(1-{2-[bis(2-{4-[({(6R)-5-(acetylamino)-3,5-dideoxy-6-[(1R,2R)-1,2,3-trihydroxypropyl]-beta-L-threo-hex-2-ulopyranonosyl}oxy)methyl]-1H-1,2,3-triazol-1-yl}ethyl)amino]ethyl}-1H-1,2,3-triazol-4-yl)methyl 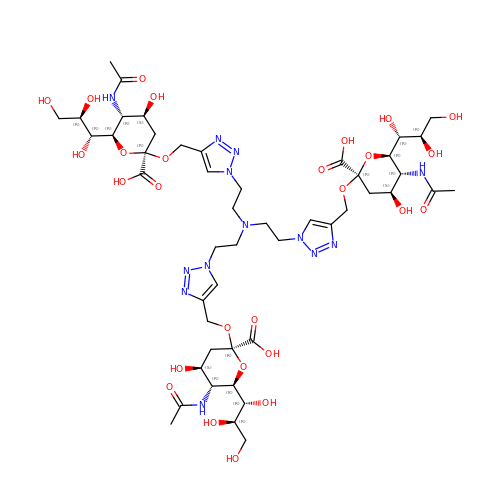(6R)-5-(acetylamino)-3,5-dideoxy-6-[(1R,2R)-1,2,3-trihydroxypropyl]-beta-L-threo-hex-2-ulopyranosidonic acid | C48 H75 N13 O27 | NXVFRYOOZMIHRF-CLUKRANESA-N> MATLGNTYLTLADVQKQKDGKGNVTSEIIEMLAETNPILEDMVVMECNDGTGHLTTIRTGLPQATWRRLYEGVQPAKSTTRQIKDSTGTLEAWSEVD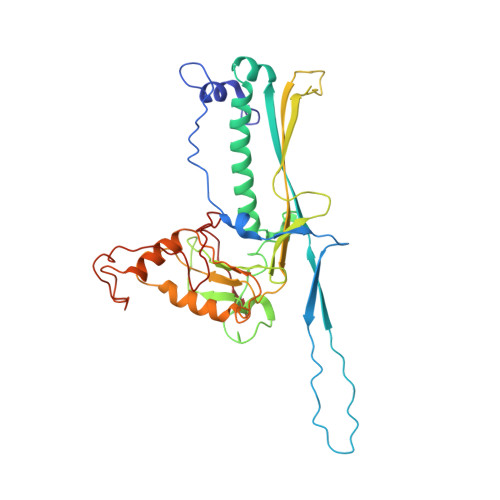EKLVKLSKDKQQLMLNEAAAFLEGMNQTMASTLFYGNTATDAVKFMGLAPRFNAYRAARNLKPVDTADQVIDAGGTGSDLTSIWMVVWGDRTAHGLYPEGTSAGLQREYLGAETKELGDGGVYRVVREKFEWDLGLTVRDFRYVVRIANIDVSDLQAGTIDIYALLRKAYYRLENRVITGGRAALYCNADVTEAMDAAATPTSSTTASYVRLTPMQVDGKEVMMYRGIPVRECDAILSTETAVPSVA> GPLGSPQMAQGTLIRVTPEQPTHAVCVLGTLTQLDICSSAPEDCTSFSINASPGVVVDIAHSPPAKKKSTGSSTWPLDPGVEVTLTMKAASGSTGDQKVQISYYGPKTPPVKALLYLTAVEISLCADITRTGKVKPTRAVKDQRTWTWGPCGQGAILLVNCDRDNLESSAMDCEDDEVLDSEDLQDMSLMTLSTKTPKDFFTNHTLVLHVARSEMDKVRVFQATRGKLSSKCSVVLGPKWPSHYLMVPGGKHNMDFYVEALAFPDTDFPGLITLTISLLDTSNLELPEAVVFQDSVVFRVAPWIMTPNTQPPQEVYACSIFENEDFLKSVTTLAMKAKCKLTICPEEENMDDQWMQDEMEIGYIQAPHKTLPVVFDSPRNRGLKEFPIKRVMGPDFGYVTRGPQTGGISGLDSFGNLEVSPPVTVRGKEYPLGRILFGDSCYPSNDSRQMHQALQDFLSAQQVQAPVKLYSDWLSVGHVDEFLSFVPAPDRKGFRLLLASPRSCYKLFQEQQNEGHGEALLFEGIKKKKQQKIKNILSNKTLREHNSFVERCIDWNRELLKRELGLAESDIIDIPQLFKLKEFSKAEAFFPNMVNMLVLGKHLGI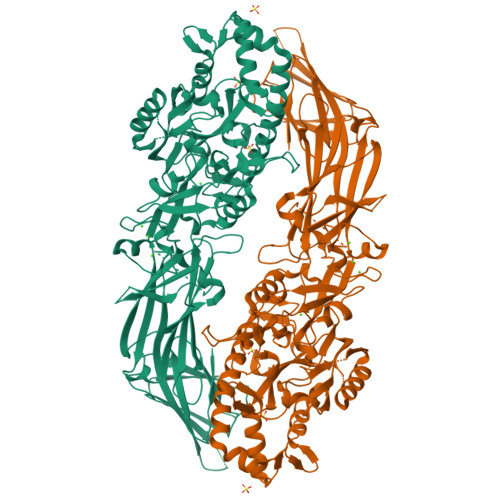PKPFGPVINGRCCLEEKVCSLLEPLGLQCTFINDFFTYHIRHGEVHAGTNVRRKPFSFKWWNMVP(2S)-2-azanyl-6-[[4-[3-(trifluoromethyl)-1,2-diazirin-3-yl]phenyl]methoxycarbonylamino]hexanoic acid | C16 H19 F3 N4 O4 | 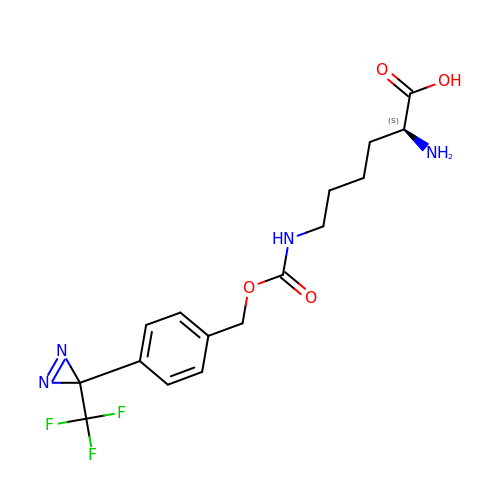MCWCMRBMGUKPHR-LBPRGKRZSA-N> MSGSLSRGNGGKKVLNKNQLLKRNRIRNARSIRAEAVAASSTKTGTPSDLSESGSKLNVDQFISSRQFEVKQLQLAMHNSKAASSTRIFQALPRKLRRRTASHNVRRIPKRMRNRALREMRKSDQQDVLKGSSASSRKAHGLNAKQLYKARMSIKLLRLASKSTSMKLSMPPEVTSSNCHVRQKIKTLKRMIKESSTANPNIKLLNNRMGSYDCTGVNELAPIPKGRVKYTKRQKHFAWLPTHIWNAKRSHMMKRWGYQMVWAPTQKCFKLTHRLGGDTCSSDGALCMDSSYIGTIIVKDKSNDSEGDFLKSIIGKLTAERANLRKYREGQVLFQGLIYSFNEENGEDSTKPLGPCDVFWVQKDTAIIRLHPSIYTQVFNILLQHKEKLTVQDCRYSLASVTLKGAKALESLASCLRSTEYSKSFEQFKMVSMITDHNALPQRCTFAFEAIDPRHLAAPKKLNDSQRKTVNSDDILSLHENYPQDEINAVFNELCDPESRTQSYNNQNTLKEISARRYKLLTATPNSINKTTVPFKESDDPSIPLVIIRRLKTRDWIVVLPWFWLLPLWHLLNRIPRMYHIGLRQFQQIQYENKQLYFPDDYPFTQLGYIENSFYKKEASKTKWDRKPMGKRINFEKIKDIHNTKLPAYSGEIGDFFSSDWRFLQILRNGIDYLQRNDKTLELMDSKKTGQFNAQGVRDINCVNDVLEFCKDYEAKTKAMSLSIEENIPVALCKNRKCQFRTPDSISVNSSSFSLTFFPRCIIAVSCTLLERGHPKDNARIYQVPEKDLEHWLQLAKGVYRPNGRKDHDLKIPLPEVHDLIGFITSGTYHLNCGNGMGIGFIDHHAAIRQPTRYVLIRNVGTNTYRLGEWSKISV;> MDRTQTFIKDCLFTKCLEDPEKPFNENRFQDTLLLLPTDGGLTSRLQRQQRKSKLNLDNLQKVSQLESADKQLEKRDYQRINKNSKIALREYINNCKKNTKKCLKLAYENKITDKEDLLHYIEEKHPTIYESLPQYVDFVPMYKELWINYIKELLNITKNLKTFNGSLALLKLSMADYNGALLRVTKSKNKTLIGLQGIVIWDSQKFFIMIVKGNIIDEIKCIPKKGTVFQFEIPISDDDDSALRYSILGDRFKYRSVDRAGRKFKSRRCDDMLYYIQN;> MVRLKSRYILFEIIFPPTDTNVEESVSKADILLSHHRASPADVSIKSILQEIRRSLSLNLGDYGSAKCNSLLQLKYFSNKTSTGIIRCHREDCDLVIMALMLMSKIGDVDGLIVNPVKVSGTIKKIEQFAMRRNSKILNIIKCSQSS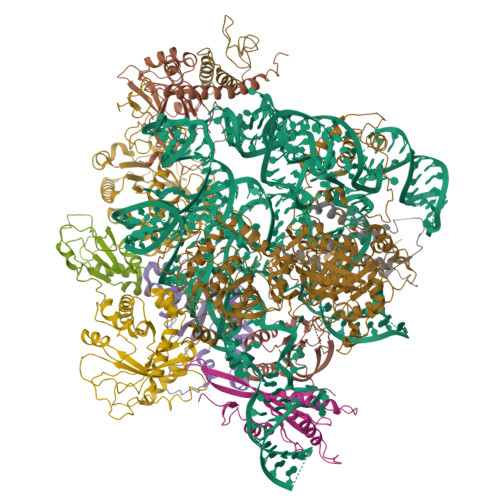HLSDNDFIINDFKKIGRENENENEDD;> MINGVYYNEISRDLDISSSTQCLRFLKETVIPSLANNGNNSTSIQYHGISKNDNIKKSVNKLDKQINMADRSLGLQQVVCIFSYGPHIQKMLSILEIFKKGYIKNNKKIYQWNKLTSFDIKREGRNELQEERLKVPILVTLVSDSEIIDLNLHSFTKQ;> MALKKNTHNKSTKRVTKHPSLKTLTHKQIHTTIFVKSTTPYVSALKRINKFLDSVHKQGSSYVAVLGMGKAVEKTLALGCHFQDQKNKKIEVYTKTIEVLDEVITEGQADIDMESDVEDDDKETQLKKRAVSGVELRIYV;> MGKKTFREWQYFKLSITSFDQDVDDAHAIDQMTWRQWLNNALKRSYGIFGEGVEYSFLHVDDKLAYIRVNHADKDTFSSSISTYISTDELVGSPLTVSILQESSSLRLLEVTDDDRLWLKKVMEEEEQDCKCI;>[2x]MLVDLNVPWPQNSYADKVTSQAVNNLIKTLSTLHMLGYTHIAINFTVNHSEKFPNDVKLLNPIDIKRRFGELMDRTGLKLYSRITLIIDDPSKGQSLSKISQAFDIVAALPISEKGLTLSTTNLDIDLLTFQYGSRLPTFLKHKSICSCVNRGVKLEIVYGYALRDVQARRQFVSNVRSVIRSSRSRGIVIGSGAMSPLECRNILGVTSLIKNLGLPSDRCSKAMGDLASLVLLNGRLRNKSHKQTIVTGGGSGNGDDVVNDVQGIDDVQTIKVVKRSMDAEQLGHASKRHKP;> MNKDQAEKYQERSLRQKYNLLHVLPTLNSRALSGLYYKNFHNSVKRYQIMLPEQLKSGKFCSHCGCVYVPNFNASLQLTTNTEQGDSDELGGESMEGPKKCIQVNCLNCEKSKLFEWKSEFVVPTFGQDVSPMINSTSSGKVSYAVKKPQKSKTSTGKERSKKRKLNSLTNLLSKRNQEKKMEKKKSSSLSLESFMKS;> MDEMDNVIRSLEQEYRLILLLNHRNKNQHRAASWYGSFNEMKRNCGQIITLFSSRRLQAKRLKDVEWVKLHRLLQRALFRQLKRWYWQFNGVIALGQFVTLGCTLVTLLANVRALYMRLWEINETEFIRCGCLIKNLPRTKAKSVVNDVEELGEIIDEDIGNNVQENELVITSIPKPLTENCKKKKKRKKKNKSAIDGIFG>[2x]MTDVIKPDYLEYDDLLDRDEMFTILEEYFMYRGLLGLRIKYGRLFNEIKKFDNDAEEQFGTIEELK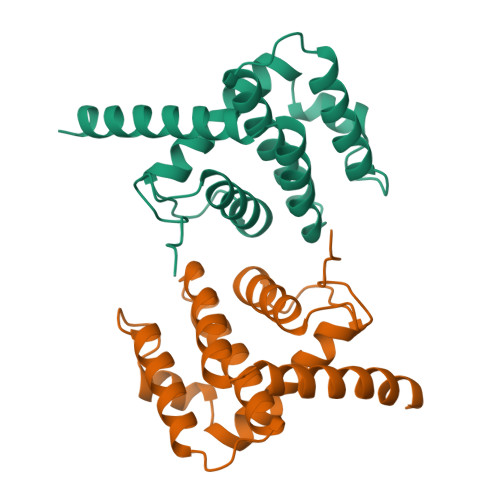QKLRLNSEEGADNFIDYIKVQKQDIVKLTVYDCISMIGLCACVVDVWRNEKLFSRWKYCLRAIKLFINDHMLDKIKSILQNRLVYVEMSKHHHHHH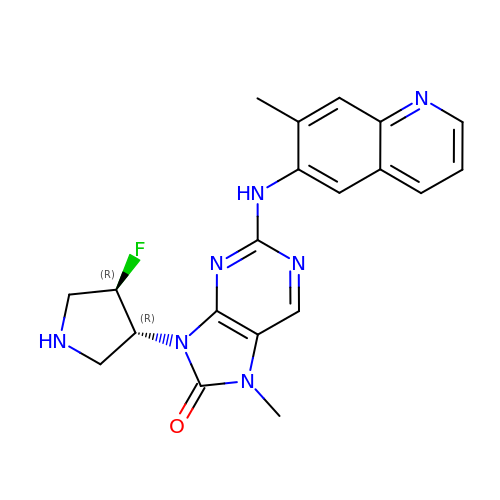9-[(3~{R},4~{R})-4-fluoranylpyrrolidin-3-yl]-7-methyl-2-[(7-methylquinolin-6-yl)amino]purin-8-one | C20 H20 F N7 O | VHGGSMHLKWIQAF-CZUORRHYSA-N> MSKQRVFIAGHRGMVGSAIRRQLEQRGDVELVLRTRDELNLLDSRAVHDFFASERIDQVYLAAAKVGGIVANNTYPADFIYQNMMIESNIIHAAHQNDVNKLLFLGSSCIYPKLAKQPMAESELLQGTLEPTNEPEAIAKIAGIKLCESYNRQYGRDYRSVMPTNLYGPHDNFHPSNSHVIPALLRRFHEATAQSAPDVVVWGSGTPMREFLHVDDMAAASIHVMELAHEVWLENTQPMLSHINVGTGVDCTIRELAQTIAKVVGYKGRVVFDASKPDGTPRKLLDVTRLH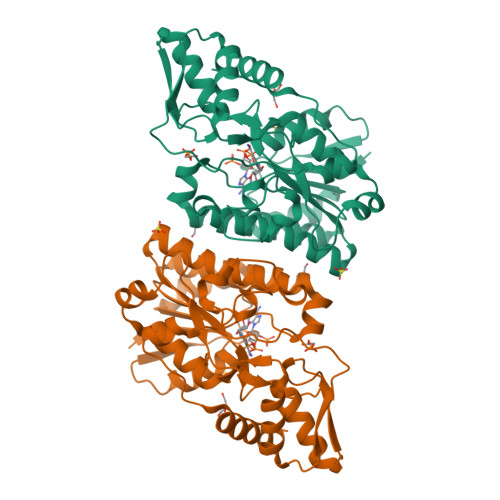QLGWYHEISLEAGLASTYQWFLENQDRFRG>AILTGVPYYILPSTSRAGFSPDNLRKNTSQPSCPLDLITQLRFPPRIGVPVIFTPQNSSLKVVPLSHNLNIHTCSDLWFCPESKIWTVKSSSIHRGLVVTTGGTFRSLGSWFRIERHG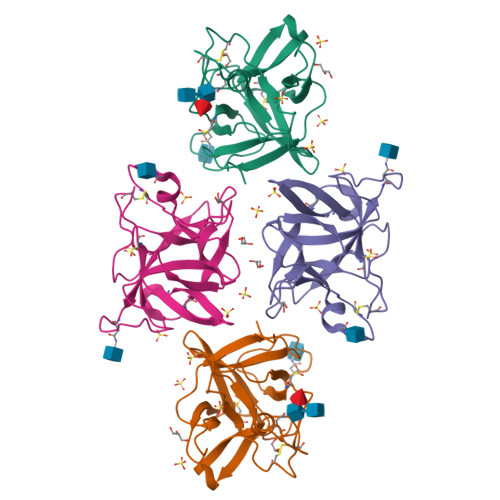DSYKLVHCPRGSTPCRDVGIETVGGGGRRYLAPRDRPLAVRFTRASG[2x]> MAAAAV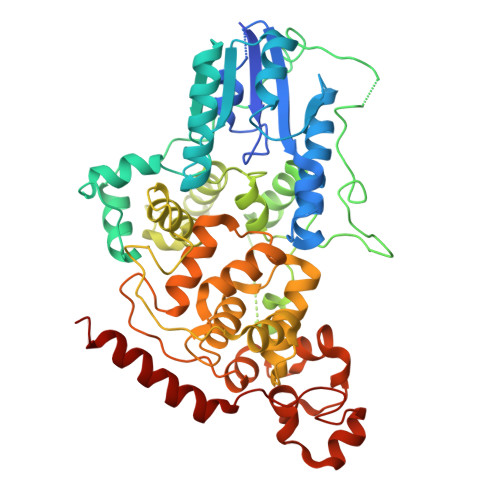VAATVPAQSMGADGASSVHWFRKGLRLHDNPALLAAVRGARCVRCVYILDPWFAASSSVGINRWRFLLQSLEDLDTSLRKLNSRLFVVRGQPADVFPRLFKEWGVTRLTFEYDSEPFGKERDAAIMKMAKEAGVEVVTENSHTLYDLDRIIELNGQKPPLTYKRFQALISRMELPKKPAVAVSSQQMESCRAEIQENHDDTYGVPSLEELGFPTEGLGPAVWQGGETEALARLDKHLERKAWVANYERPRMNANSLLASPTGLSPYLRFGCLSCRLFYYRLWDLYKKVKRNSTPPLSLFGQLLWREFFYTAATNNPRFDRMEGNPICIQIPWDRNPEALAKWAEGKTGFPWIDAIMTQLRQEGWIHHLARHAVACFLTRGDLWVSWESGVRVFDELLLDADFSVNAGSWMWLSCSAFFQQFFHCYCPVGFGRRTDPSGDYIRRYLPKLKGFPSRYIYEPWNAPESVQKAAKCIIGVDYPRPIVNHAETSRLNIERMKQIYQQLSRY2-{[4-amino-3-(3-fluoro-5-hydroxyphenyl)-1H-pyrazolo[3,4-d]pyrimidin-1-yl]methyl}-5-methyl-3-(2-methylphenyl)quinazolin-4(3H)-one | C28 H22 F N7 O2 | 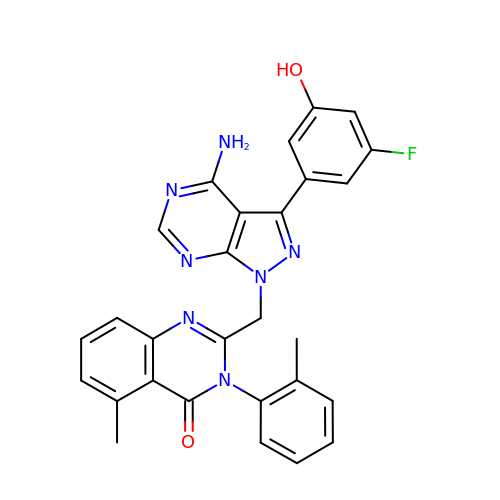AUNMZFMPIXHYCD-UHFFFAOYSA-N>[4x]MVSANGDLHLPISNEQCMPENNGSLGFEAPTPDRFDRDRLFSVVSRGVPEELTGLLEYLRWNSKYLTDSAYTEGSTGKTCLMKAVLNLQDGVNACIMPLLQIDKDSGNPKPLVNAQCTDEFYQGHSALHIAIEKRSLQCVKLLVENGADVHLRA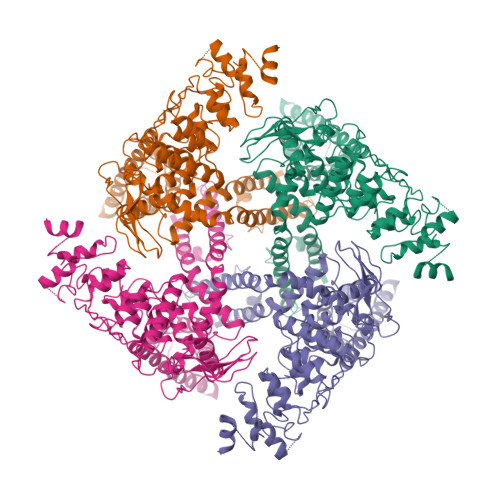CGRFFQKHQGTCFYFGELPLSLAACTKQWDVVTYLLENPHQPASLEATDSLGNTVLHALVMIADNSPENSALVIHMYDGLLQMGARLCPTVQLEEISNHQGLTPLKLAAKEGKIEIFRHILQREFSGPYQPLSRKFTEWCYGPVRVSLYDLSSVDSWEKNSVLEIIAFHCKSPNRHRMVVLEPLNKLLQEKWDRLVSRFFFNFACYLVYMFIFTVVAYHQPSLDQPAIPSSKATFGESMLLLGHILILLGGIYLLLGQLWYFWRRRLFIWISFMDSYFEILFLLQALLTVLSQVLRFMETEWYLPLLVLSLVLGWLNLLYYTRGFQHTGIYSVMIQKVILRDLLRFLLVYLVFLFGFAVALVSLSREARSPKAPEDNNSTVTEQPTVGQEEEPAPYRSILDASLELFKFTIGMGELAFQEQLRFRGVVLLLLLAYVLLTYVLLLNMLIALMSETVNHVADNSWSIWKLQKAISVLEMENGYWWCRRKKHREGRLLKVGTRGDGTPDERWCFRVEEVNWAAWEKTLPTLSEDPTETSQVAPA>MAHHHHHHMKILLIGKNGQVGWELQRSLSTLGDVVAVD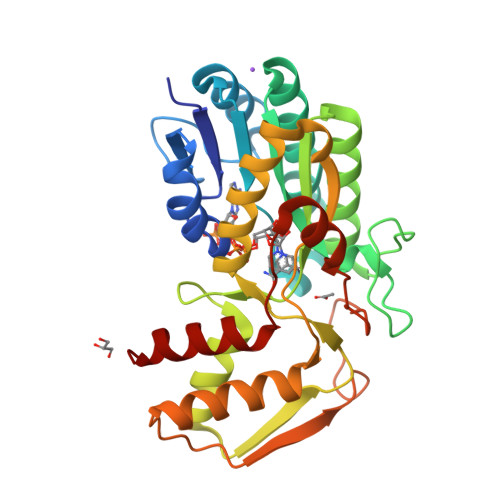YFDKELCGDLTNLDGIAQTVRTVRPDVVVNAAAHTAVDKAESERELSDLLNDKGVAVLAAESAKLGALMVHYSTDYVFDGAGSHYRREDEATGPLNVYGETKRAGELALEQGNPRHLIFRTSWVYATRGANFAKTMLRLAGEKETLSIIDDQHGAPTGAELLADCTATAIRETLRDPALAGTYHLVASGETSWCDYARYVFEVARAHGAELAVQEVKGIPTTAYPTPAKRPLNSRLSNEKFQQAFGVTLPDWRQGVARVVTEVLGK[4x]> SMAFLILVIGNLHIPDRALDIPPKFKKLLSPGKI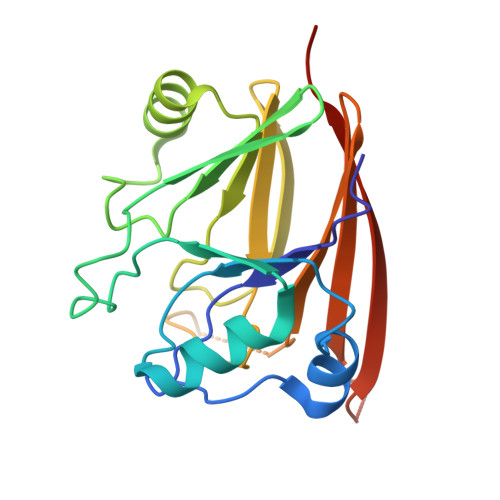SQTLCLGNLTDRATYDYLRSISPDLKIVRGRMDVEATSLPLMQVVTHGSLRIGFLEGFTLVSEEPDVLLAEANKLDVDVLCWAGGSHRFECFEYMDKFFVNPGSATGAFTTDWLAEGEEVVPSFCLMDVQGISLTLYVYQLRKDENGTENVAVEKVTYTKPVEPTGAS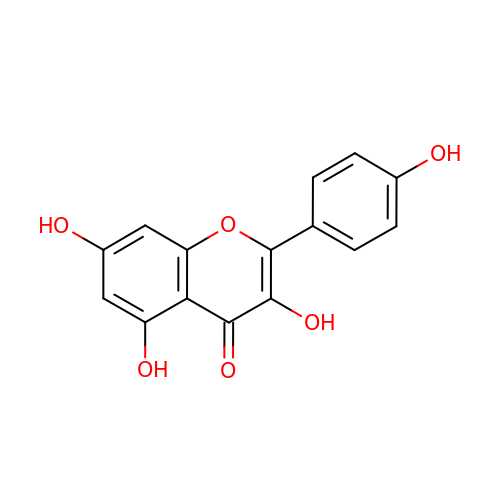3,5,7-TRIHYDROXY-2-(4-HYDROXYPHENYL)-4H-CHROMEN-4-ONE | C15 H10 O6 | IYRMWMYZSQPJKC-UHFFFAOYSA-N> MTDRY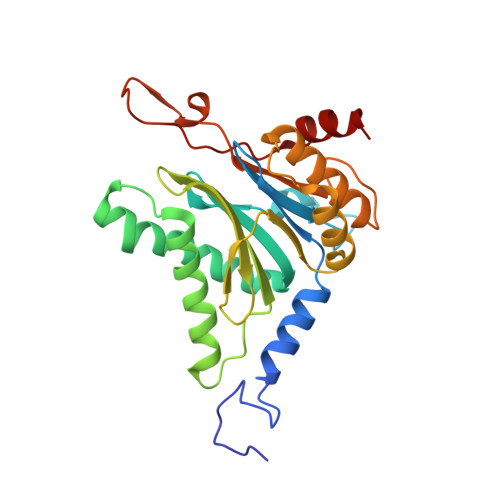SFSLTTFSPSGKLGQIDYALTAVKQGVTSLGIKATNGVVIATEKKSSSPLAMSETLSKVSLLTPDIGAVYSGMGPDYRVLVDKSRKVAHTSYKRIYGEYPPTKLLVSEVAKIMQEATQSGGVRPFGVSLLIAGHDEFNGFSLYQVDPSGSYFPWKATAIGKGSVAAKTFLEKRWNDELELEDAIHIALLTLKESVEGEFNGDTIELAIIGDENPDLLGYTGIPTDKGPRFRKLTSQEINDRLEAL>[6x]SNAM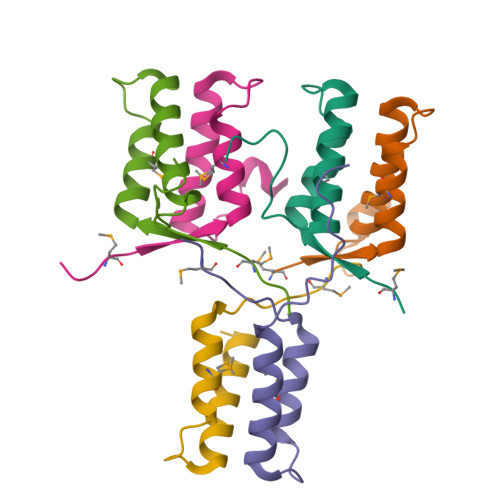KYFQIDELTLNAMLRITTIESLTPEQRLELIKAHLLNIKTPSDDNEPWDEF> QSAPHDLPEGFEFMEHKVVN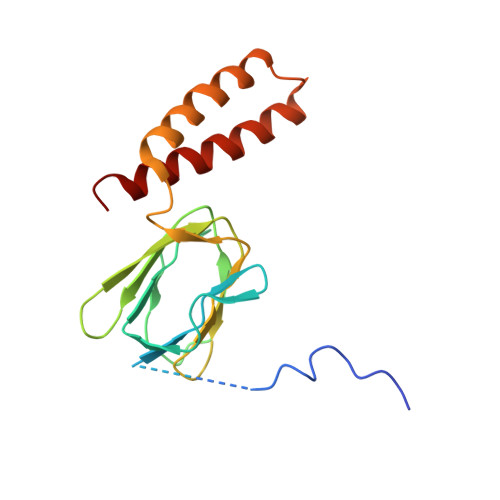KDIHAPHENLETLRLTLTRQDEFLLREEPVKCVTVTGTNGEYGIYPGHAYKIVQLNPSPLTVEYTDGTTKKYFVSGGFAHINNEGSCDVNTVECTLLDDLDLAIAEKELAAQQAALGSAKDDKAKSVVEIRISVIEAVIAALKHH>SMSNRLIFDADWLVPEQVQVAGQAIQYYAARNIQYVQHPVAAIQVLNVFVPAAYLHGSSVNGYQRATAPILMPNTVGGYLPGPADDPQRVTWPTNAGTIQQALKRGYVVVAAGIRGRTTVDKSGQRVGQAPAFIVDMKAAIRYVKYNQGRLPGDANRIITNGTSAGGATSALAGASGNSAYFEPALTALGAAPATDDIFAVSAYCPIHNLEHADMAYEWQFNGINDWHRYQPVAGTTKNGRPKFEPVSGQLTVEEQALSLALKAQFSTYLNQLKLTASDGTHLTLNEAGMGSFRDVVRQLLISSAQTAFDQGTDIHKYAGFVVTGNQVTDLDLSAYLKSLTRMKAVPAFDQLDLTSPENNLFGDATAKAKHFTALAQTRSTVTAQLADAELIQAINPLSYLTTTSSQVAKHWRIRHGAA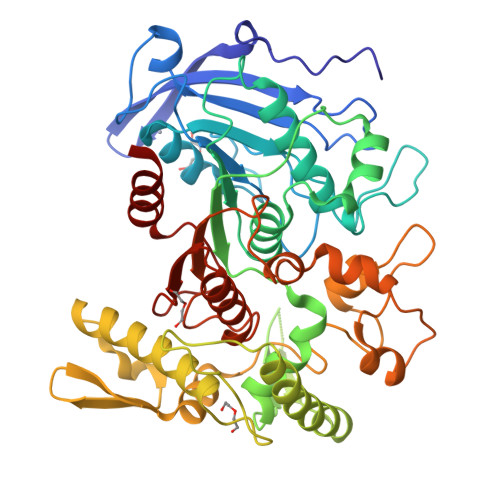DRDTSFAIPIILAIMLENHGYGIDFALPWDIPHSGDYDLGDLFSWIDGLCQ[2x]> MKGFAMLGINKLGWIEKERPVAGSYDAIVRPLAVSPCTSDIHTVFEGALGDRKNMILGHEAVGEVVEVGSEVKDFKPGDRVIVPCTTPDWRSLEVQAGFQQHSNGMLAGWKFSNFKDGVFGEYFHVNDADMNLAILPKDMPLENAVMITDMMTTGFHGAELADIELGATVAVLGIGPVGLMAVAGAKLRGAGRIIAVGSRPVCVDAAKYYGATDIVNYKDGPIESQIMNLTEGKGVDAAIIAGGNADIMATAVKIVKPGGTIANVNYFGEGEVLPVPRLEWGCGMAHKTIKGGLCPGGRLRAEMLRDMVVYNRVDLSKLVTHVYHGFDHI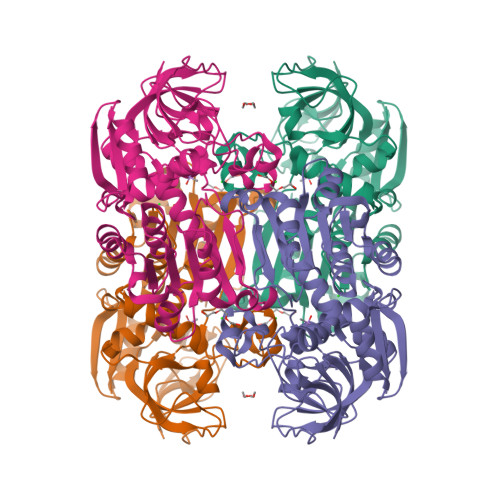EEALLLMKDKPKDLIKAVVIL> AYLQDMPRSPGDVPQSPSDVSPSPDAPQSPGGMPHLPGDVLHSPGDMPHSSGDVTHSPRDIPHLPGDRPDFTQNDVQNRDMPMDISALSSPSCSPRPQSETPLEKVPWLSVMETPARKEISLSEPAKPGSAHVQSRTPQ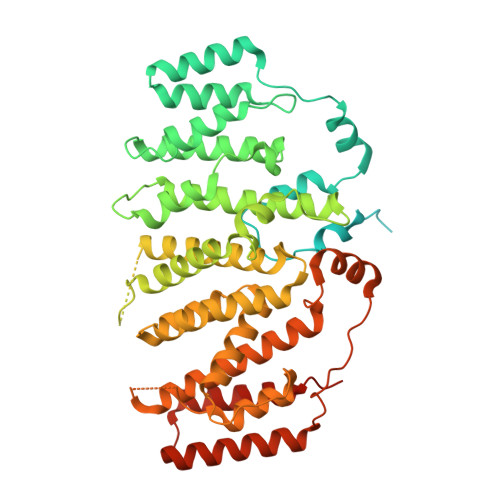GGLYNRPCLHRLKYFLRPPVHHLFFQTLIPDKDTRENKGQRLEPIPHRRLRMVTNTIEENFPLGTVQFLMDFVSPQHYPPREIVAHIIQKILLSGSETVDVLKEAYMLLMKIQQLHPANAKTVEWDWKLLTYVMEEEGQTLPGRVLFLRYVVQTLEDDFQQTLRRQRQHLQQSIANMVLSCDKQPHNVRDVIKWLVKAVTEDGLTQPPNGNQTSSGTGILKASSSHPSSQPNLTKNTNQLIVCQLQRMLSIAVEVDRTPTCSSNKIAEMMFGFVLDIPERSQREMFFTTMESHLLRCKVLEIIFLHSCETPTRLPLSLAQALYFLNNSTSLLKCQSDKSQWQTWDELVERLQFLLSSYQHVLREHLRSSVIDRKDLIIKRIKPKPQQGDDITVVDVEKQIEAFRSRLIQMLGEPLVPQLQDKVHLLKLLLFYAADLNPDAEPFQKGWSGS> MRKISLIILLLFLQNGFSQETKPRFNYNAKYEPQTGIYHGAGQDKNGFQDYVNAVGQDKMPAIYMTYVNITAPVKRIESWGKDLKHVLDSLPKGIMPQIGLAFTGGKDTGAGLDKEVANGKYNAQLEAFYKVLLDLDRPSFTRIGYEFEGDWNGYSPESFKKVFITISKAFEEKNIKSATVWCSGGGSANFIGLEKLMAYYPG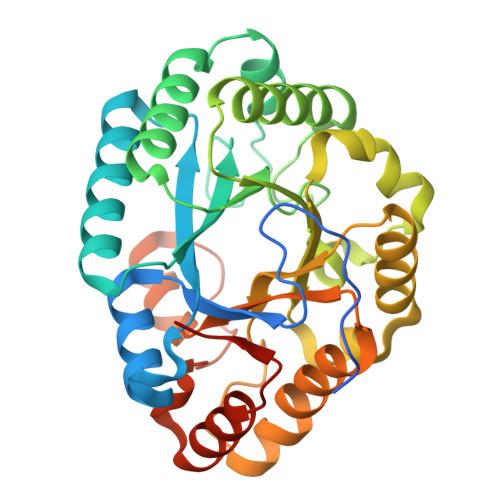NEYVDWWGIDVFSPEEFSNIGLKNFFDTAHTHKKPVMIGESTPRYVGVLDGEISWNKWFKPFFEMLNDNPGIKAFCYINWDWEYWSNKNGFPWHDWKDARIEKNPFVLEAYKTEMENPIFIHLNNKLEHHHHHH> MSSEQLHEPAELLSEETKNMHRALVTLIEELEAVDWYQQRADACSEPGLHDVLIHNKNEEVEHAMMTLEWIRRRSPVFDAHMRTYLFTERPI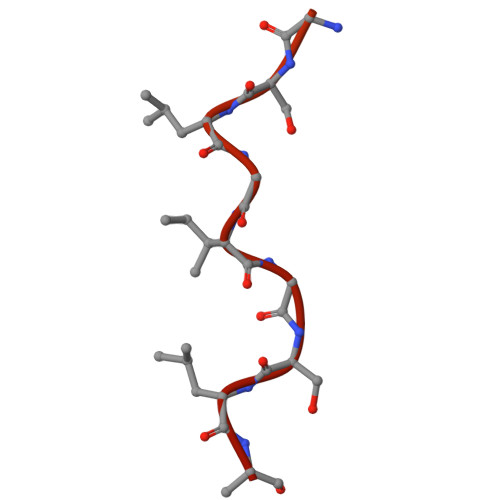LELEEEDTGSSSSVAASPTSAPSHGSLGIGSLRQEGKED> MPAPLYGADDPRRCSGNSVSEVLDKFRKNYDLIMSLPQETKEEKEFRHCIWLAEKEERERIYQTAIRPFRKATYTKFIEIDPRLRDYRSRYAGISNN;> MSDVAETLDPLRLPLQGERLIEASAGTGKTFTIAALYLRLLLGLGGSAAFPRPLTVEELLVVTFTEAATAELRGRIRSNIHELRIACLRETTDNPLYERLLEEIDDKAQAAQWLLLAERQMDEAAVFTIHGFCQRMLNLNAFESGMLFEQQLIEDESLLRYQACADFWRRHCYPLPREIAQVVFETWKGPQALLRDINRYLQGEAPVIKAPPPDDETLASRHAQIVARIDTVKQQWRDAVGELDALIESSGIDRRKFNRSNQAKWIDKISAWAEEETNSYQLPESLEKFSQRFLEDRTKAGGETPRHPLFEAIDQLLAEPLSIRDLVITRALAEIRETVAREKRRRGELGFDDMLSRLDSALRSESGEVLAAAIRTRFPVAMIDEFQDTDPQQYRIFRRIWHHQPETALLLIGDPKQAIYAFRGADIFTYMKARSEVHAHYTLDTNWRSAPGMVNSVNKLFSQTDDAFMFREIPFIPVKSAGKNQALRFVFKGETQPAMKMWLMEGESCGVGDYQSTMAQVCAAQIRDWLQAGQRGEALLMNGDDARPVRASDISVLVRSRQEAAQVRDALTLLEIPSVYLSNRDSVFETLEAQEMLWLLQAVMTPERENTLRSALATSMMGLNALDIETLNNDEHAWDVVVEEFDGYRQIWRKRGVMPMLRALMSARNIAENLLATAGGERRLTDILHISELLQEAGTQLESEHALVRWLSQHILEPDSNASSQQMRLESDKHLVQIVTIHKSKGLEYPLVWLPFITNFRVQEQAFYHDRHSFEAVLDLNAAPESVDLAEAERLAEDLRLLYVALTRSVWHCSLGVAPLVRRRGDKKGDTDVHQSALGRLLQKGEPQDAAGLRTCIEALCDDDIAWQTAQTGDNQPWQVNDVSTAELNAKTLQRLPGDNWRVTSYSGLQQRGHGIAQDLMPRLDVDAAGVASVVEEPTLTPHQFPRGASPGTFLHSLFEDLDFTQPVDPNWVREKLELGGFESQWEPVLTEWITAVLQAPLNETGVSLSQLSARNKQVEMEFYLPISEPLIASQLDTLIRQFDPLSAGCPPLEFMQVRGMLKGFIDLVFRHEGRYYLLAYKSNWLGEDSSAYTQQAMAAAMQAHRYDLQYQLYTLALHRYLRHRIADYDYEHHFGGVIYLFLRGVDKEHPQQGIYTTRPNAGLIALMDEMFAGMTLEEA;> MLRVYHSNRLDVLEALMEFIVERERLDDPFEPEMILVQSTGMAQWLQMTLSQKFGIAANIDFPLPASFIWDMFVRVLPEIPKESAFNKQSMSWKLMTLLPQLLEREDFTLLRHYLTDDSDKRKLFQLSSKAADLFDQYLVYRPDWLAQWETGHLVEGLGEAQAWQAPLWKALVEYTHQLGQPRWHRANLYQRFIETLESATTCPPGLPSRVFICGISALPPVYLQALQALGKHIEIHLLFTNPCRYYWGDIKDPAYLAKLLTRQRRHSFEDRELPLFRDSENAGQLFNSDGEQDVGNPLLASWGKLGRDYIYLLSDLESSQELDAFVDVTPDNLLHNIQSDILELENRAVAGVNIEEFSRSDNKRPLDPLDSSITFHVCHSPQREVEVLHDRLLAMLEEDPTLTPRDIIVMVADIDSYSPFIQAVFGSAPADRYLPYAISDRRARQSHPVLEAFISLLSLPDSRFVSEDVLALLDVPVLAARFDITEEGLRYLRQWVNESGIRWGIDDDNVRELELPATGQHTWRFGLTRMLLGYAMESAQGEWQSVLPYDESSGLIAELVGHLASLLMQLNIW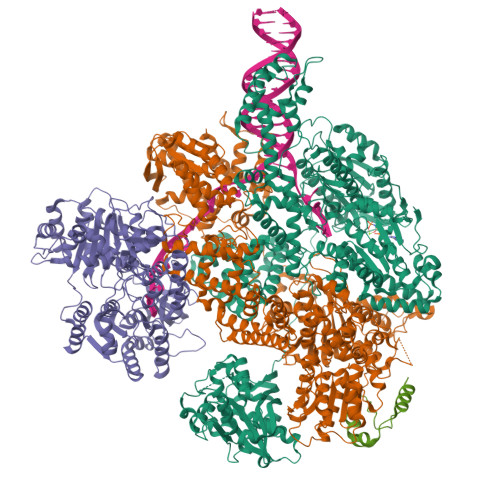RRGLAQERPLEEWLPVCRDMLNAFFLPDAETEAAMTLIEQQWQAIIAEGLGAQYGDAVPLSLLRDELAQRLDQERISQRFLAGPVNICTLMPMRSIPFKVVCLLGMNDGVYPRQLAPLGFDLMSQKPKRGDRSRRDDDRYLFLEALISAQQKLYISYIGRSIQDNSERFPSVLVQELIDYIGQSHYLPGDEALNCDESEARVKAHLTCLHTRMPFDPQNYQPGERQSYAREWLPAASQAGKAHSEFVQPLPFTLPETVPLETLQRFWAHPVRAFFQMRLQVNFRTEDSEIPDTEPFILEGLSRYQINQQLLNALVEQDDAERLFRRFRAAGDLPYGAFGEIFWETQCQEMQQLADRVIACRQPGQSMEIDLACNGVQITGWLPQVQPDGLLRWRPSLLSVAQGMQLWLEHLVYCASGGNGESRLFLRKDGEWRFPPLAAEQALHYLSQLIEGYREGMSAPLLVLPESGGAWLKTCYDAQNDAMLDDDSTLQKARTKFLQAYEGNMMVRGEGDDIWYQRLWRQLTPETMEAIVEQSQRFLLPLFRFNQS;> MKLQKQLLEAVEHKQLRPLDVQFALTVAGDEHPAVTLAAALLSHDAGEGHVCLPLSRLENNEASHPLLATCVSEIGELQNWEECLLASQAVSRGDEPTPMILCGDRLYLNRMWCNERTVARFFNEVNHAIEVDEALLAQTLDKLFPVSDEINWQKVAAAVALTRRISVISGGPGTGKTTTVAKLLAALIQMADGERCRIRLAAPTGKAAARLTESLGKALRQLPLTDEQKKRIPEDASTLHRLLGAQPGSQRLRHHAGNPLHLDVLVVDEASMIDLPMMSRLIDALPDHARVIFLGDRDQLASVEAGAVLGDICAYANAGFTAERARQLSRLTGTHVPAGTGTEAASLRDSLCLLQKSYRFGSDSGIGQLAAAINRGDKTAVKTVFQQDFTDIEKRLLQSGEDYIAMLEEALAGYGRYLDLLQARAEPDLIIQAFNEYQLLCALREGPFGVAGLNERIEQFMQQKRKIHRHPHSRWYEGRPVMIARNDSALGLFNGDIGIALDRGQGTRVWFAMPDGNIKSVQPSRLPEHETTWAMTVHKSQGSEFDHAALILPSQRTPVVTRELVYTAVTRARRRLSLYADERILSAAIATRTERRSGLAALFSSRE>G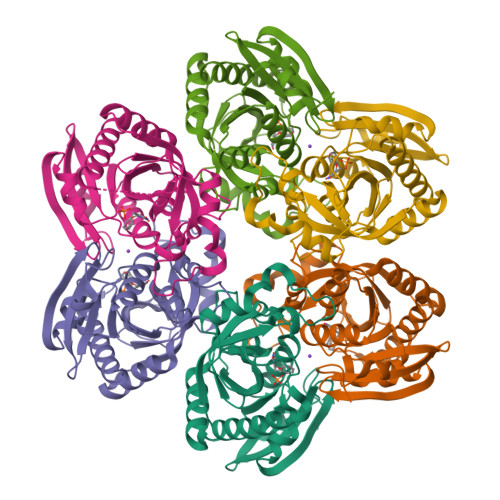SHMSKSDVFHLGLTKNDLQGATLAIVPGDPDRVEKIAALMDKPVKLASHREFTTWRAELDGKPVIVCSTGIGGPSTSIAVEELAQLGIRTFLRIGTTGAIQPHINVGDVLVTTASVRLDGASLHFAPLEFPAVADFECTTALVEAAKSIGATTHVGVTASSDTFYPGQERYDTYSGRVVRHFKGSMEEWQAMGVMNYEMESATLLTMCASQGLRAGMVAGVIVNRTQQEIPNAETMKQTESHAVKIVVEAARRLL[6x]> MAGVEEVAASGSHLNGDLDPDDREEGAASTAEEAAKKKRRKKKKSKGPSAAGEQEPDKESGASVDEVARQLERSALEDKERDEDDEDGDGDGDGATGKKKKKK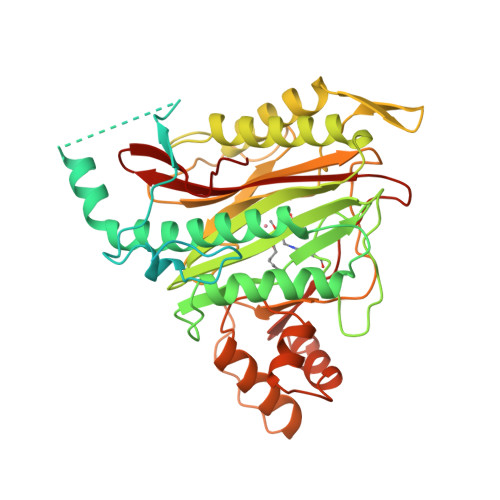KKKRGPKVQTDPPSVPICDLYPNGVFPKGQECEYPPTQDGRTAAWRTTSEEKKALDQASEEIWNDFREAAEAHRQVRKYVMSWIKPGMTMIEICEKLEDCSRKLIKENGLNAGLAFPTGCSLNNCAAHYTPNAGDTTVLQYDDICKIDFGTHISGRIIDCAFTVTFNPKYDTLLKAVKDATNTGIKCAGIDVRLCDVGEAIQEVMESYEVEIDGKTYQVKPIRNLNGHSIGQYRIHAGKTVPIVKGGEATRMEEGEVYAIETFGSTGKGVVHDDMECSHYMKNFDVGHVPIRLPRTKHLLNVINENFGTLAFCRRWLDRLGESKYLMALKNLCDLGIVDPYPPLCDIKGSYTAQFEHTILLRPTCKEVVSRGDDY>VETPPEVVDFMVSLAEAPRGGRVLEPACAHGPFLRAFREAHGTGYRFVGVEIDPKALDLPPWAEGILADFLLWEPGEAFDLILGNPPYGIVGEASKYPIHVFKAVKDLYKKAFSTWKGKYNLYGAFLEKAVRLLKPGGVLVFVVPATWLVLEDFALLREFLAREGKTSVYYLGEVFPQKKVSAVVIRFQKSGKGLSLWDTQESESGFTPILWAEYPHWEGEIIRFETEETRKLEISGMPLGDLFHIRFAARSPEFKKHPAVRKEPGPGLVPVLTGRNLKPGWVDYEKNHSGLWMPKERAKELRDFYATPHLVVAHTKGTRVVAAWDE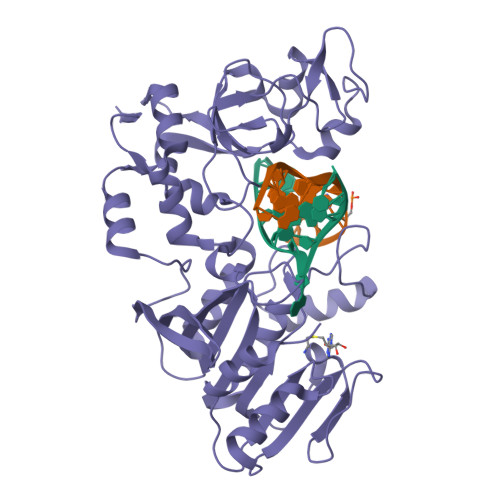RAYPWREEFHLLPKEGVRLDPSSLVQWLNSEAMQKHVRTLYRDFVPHLTLRMLERLPVRREYGFHT[2x]4-[(6,7-dimethoxy-2,4-dihydroindeno[1,2-c]pyrazol-3-yl)ethynyl]-2-methoxyphenol | C21 H18 N2 O4 | 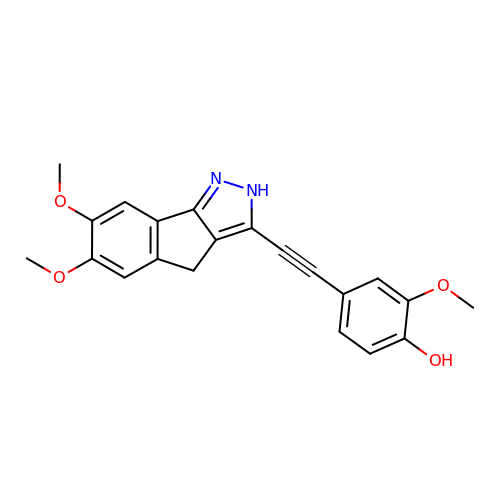MPWLZTAOZDBWMH-UHFFFAOYSA-N>[2x]MRILHSMLRVADLEAALEFYTRALDMRLLRRRDYPEGRFTLAFVGYQDERAAAALELTHN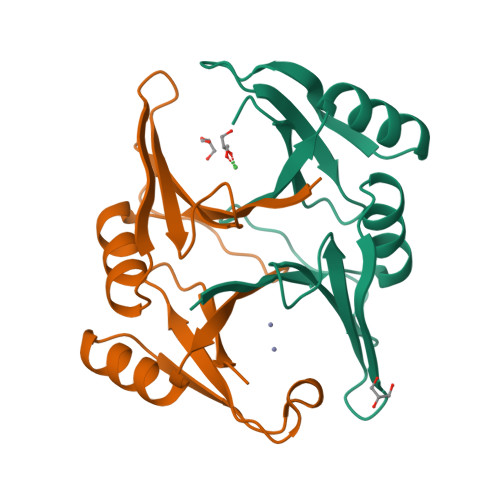WDRDGYTQGDGYGHLAIEVEDAAVTCARARALGYRVTREAGLMQHGRSVIAFLEDPDGYKVELIQKGTQFD> MASHHLSWLHEINSQELEKAHATLLGLANMETRYFAKKKTLLGLSKLAALASDFSEDMLQEKIEEMAEQERFLLHQETLPEQLLAEKQLNLSAMPVLTAPQLIGLYICEENRRANEYDFKKALDLLEYIDEEEDININDLKLEILCKALQRDNWSSSDGKDDPIEVSKDSIFVK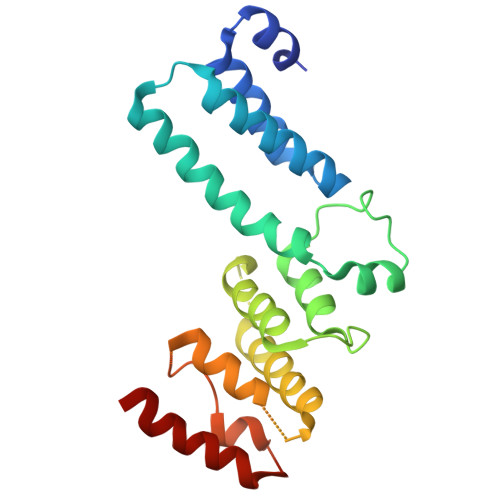ILQKLLKDGIQLSEYLPEVKDLLQADQLGSLKSNPYFEFVLKANYEYYVQGQI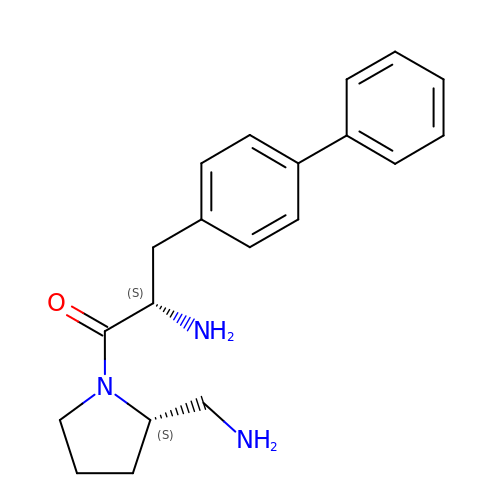1-[2-(S)-AMINO-3-BIPHENYL-4-YL-PROPIONYL]-PYRROLIDINE-2-(S)-CARBONITRILE | C20 H25 N3 O | MUUVLSCVDXKQQV-OALUTQOASA-N> SKDRDLSKVSPYENIPAKGFTHGVGFDYGVPLSLFPDNAIDPTIANPESIDEMSIQYLASRPYMLDRYTIKGGNTPSPSGTVVADIPISPVNYSLYGSIIRDYRTIFGAPVSLAVAMASWWRAKIHLNLQFAKTQYHQCRLLVQYLPYGSDVQSLENVLSQIIDISHVDESGIDLCFPSIFTNKWMRSYDPATE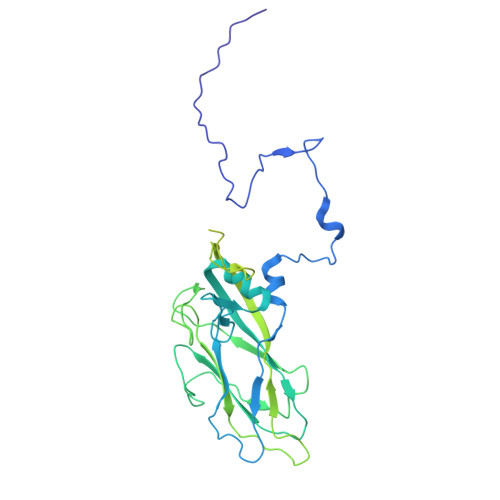GYTAGCAPGRILISVLNPLISASTVNDDIVMMPWLTWENLELAEPGSLAKAAIGFDYPADAVDEKWTSRELPVTGSSFNLFRDTTIVLGASTNISNLVLTNDDTGGDYQIVSTTPTGSYVSAVTCPQGTYTITHDGVGATIISNFPILGAGEGPSFQISALRHGDKVTITEDPTKINVSGVSFLTGTNSWKASLKDSSGTLLGRLEYDGTSFSSDSPASLIPGKYNVELDPADNSAVVTIVANNSFGTASLDTH> CQPIFLNVLEAIEPG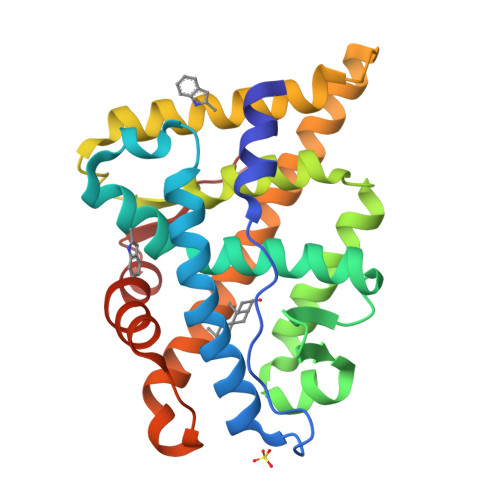VVCAGHDNNQPDSFAALLSSLNELGERQLVHVVKWAKALPGFRNLHVDDQMAVIQYSWMGLMVFAMGWRSFTNVNSRMLYFAPDLVFNEYRMHKSRMYSQCVRMRHLSQEFGWLQITPQEFLCMKALLLFSIIPVDGLKNQKFFDELRMNYIKELDRIIACKRKNPTSCSRRFYQLTKLLDSVQPIARELHQFTFDLLIKSHMVSVDFPEMMAEIISVQVPKILSGKVKPIYFHTQ> GIDPFYMGGDGKSDGAGDGSGGAAKSGPWSFKDDRGTTVKLDKVPANIVAFTGVAAALFDYGVEVKGVFGPTTTKDGKPDVQAGDLDVDKVTVLGNEWGKLNVEKYASLAPEVLITTTFDTAGTLWSVPEESKDKVAKLAPSVAISVFDRQLTQPLQRMWELAESLGADMKAKKVTDAKAAFDKAAARLRAAAKAKPEIRVLAGSASPDLFYVSGTNLSVDLEYFKALGVNFVEPSEDAKKATGGWFES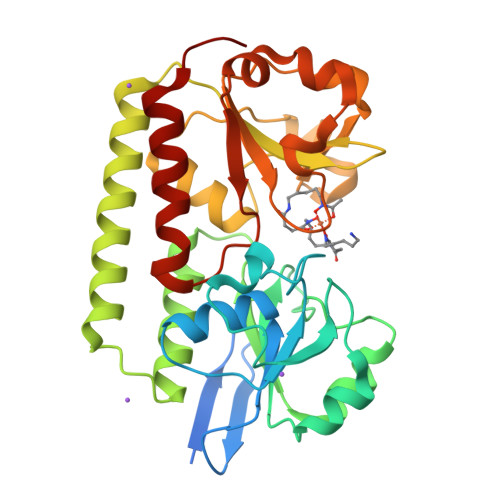LSWENVDKYPADVIIMDDRASTIQPADITEGTWKQLPAVKAGQVIARSPEPILSYDKCTPLLDNLAEAIENAKKVG>ATKKAVAVLKGNSNVEGVVTLSQDDDGPTTVNVRITGLAPGLHGFHLHEYGDTTNGCMSTGAHFNPNKLTHGAPGDEIRHAGDLGNIVAN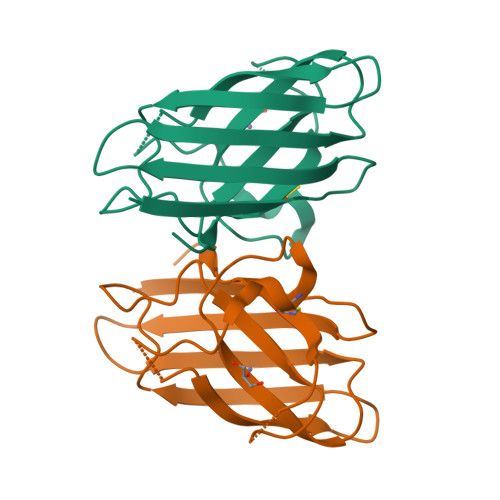ADGVAEVTLVDNQIPLTGPNSVVGRALVVHELEDDLGKGGHELSLTTGNAGGRLACGVVGLTPI[2x]> GPGHMELSLRNVAKIVEQIDRAVYSIDLAIYTFTSLFLADSIKRALQRGVIIRIISDGEMVYSKGSQISMLAQLGVPVRVPITTNLMHNKFCIIDGFERVEEIRLLRKLKFMRPCYSIVISGSVNWTALGLGGNWENCIITADDKL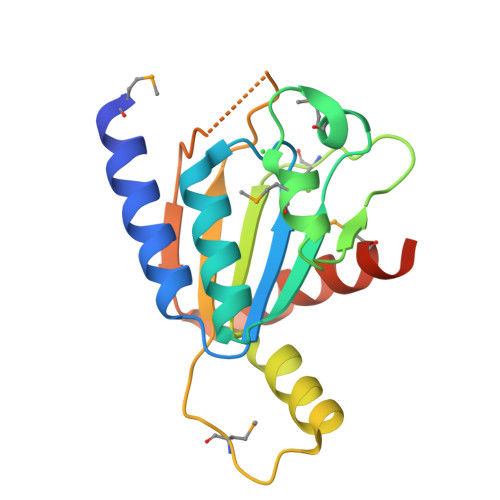TATFQAEFQRMWRAFAKTEGSQI>MPVTNMAELDAMIARVKKAQEEFATYSQEQVDKIFRAASLAANQARIPLAQQAVEESGMGIVEDKVIKNHFASEFIYNKYKDEQTCGILEEDDNLGTMTIAEPVGIICGIVPTTNPTSTAIFKSLISLKTRNGIIFSPHPRAKNSTNDAAKLVLDAAVAAGAPKDIIGWIDQPSVELSNALMKHDDIALILATGGPGMVKAAYSSGKPAIGVGAGNVPVVIDETADIKRAVASVLMSKTFDNGVVCASEQAVIVVDEVYDEVKERFASHKAHVLSKTDADKV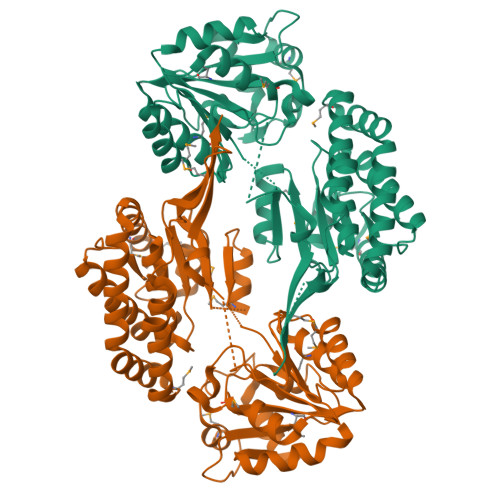RKVLLIDGALNAKIVGQPATAIAEMAGVKVPADTKVLIGEGLGKVSYDDAFAHEKLSPTLGMFRADNFEDAVAQAVTMVEIGGIGHTSGLYTNQDVNADRIRYFGDKMKTARILINIPTTHGGIGDLYNFNVAPSLTLGCGSWGGNSISENVGPKHLINKKTVAKRAENM[4x]>MQMNSEKFFKLFRVGETVLVEYSGTSRAELLLYYIVNNSKLPIVVDDILDTYYEFYTRLKVAGFDVAPLENVQVIKMGGTKDIGRVIGRLNISKYVISEQEYMEIVSQLKDYPVINPVLGLHKLILLGN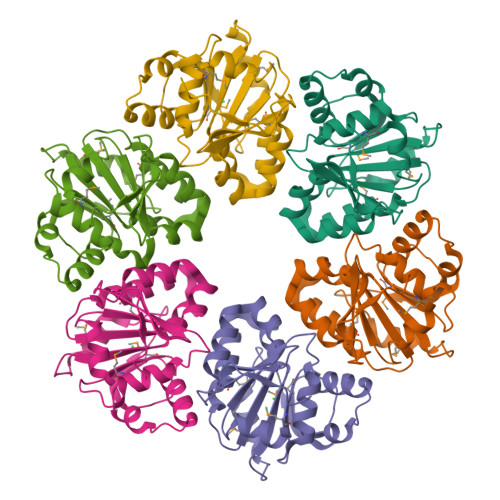TFENINVVKMVSNYVGREERIAFYFVNRNVIEKHSSPILDLLEEVVTSILEITDSGIIIKKSIKDEIAGKIVSPLLNF[6x]2,4-dihydroxy-3,6-dimethylbenzaldehyde | C9 H10 O3 | 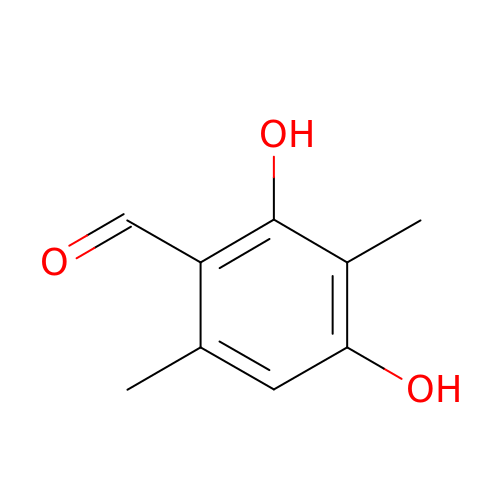XOAAGSCMGLMPKG-UHFFFAOYSA-N> GASETQQWKTLEDTRSALMGVYGLTRAALADNNTHWICGDLRKGDFTVYKRSDLQAVSDNELNKPYDLLKKVSNWRRFYAVINAASVFMEKAPRTVELDRSYSEQNLKYDIAQVRALRAFAYFYMVRIWGDVPLVTYSYDNGTFPSMPRTDAQTVLSYAKAELLTAIEDLPYQYGTQTNLYYGSYGAQWQGKLFNKLSAYSVLAHICAWQGNYAEAETYSAFIIDHASEINAKYTSIADLTSETGLFYSNASVKGSRILGFNFAHNDNEATQSGHLEQLTLAYPLVQKSYPEIYISKDSLFSIFTNFDDLRFGIIDTIKYSSYYVQNLNEETPVFSKIKIIQDGSAKDNDFGVFGSSIVFTRL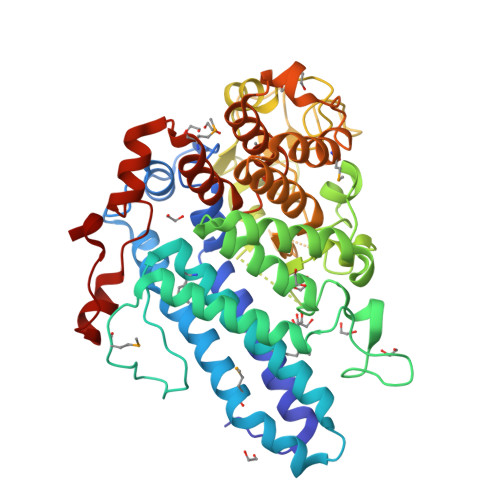EDITLLRAEALCALNRSTEAVSYLNMIRTNRGLREVSFKKDFGNNRESLIAEIFEERRRELMGEGWRWYDLVRRQKLMKDNEAFLRLISSGGIYWPVSEDIITANSQIEQNEFWK> QPVNHLVKEIDMLLKEYLLSGDISEAEHCLKELEVPHFHHELVYEAIVMVLESTGESAFKMILDLLKSLWKSSTITIDQMKRGYERIYNEIPDINLDVPH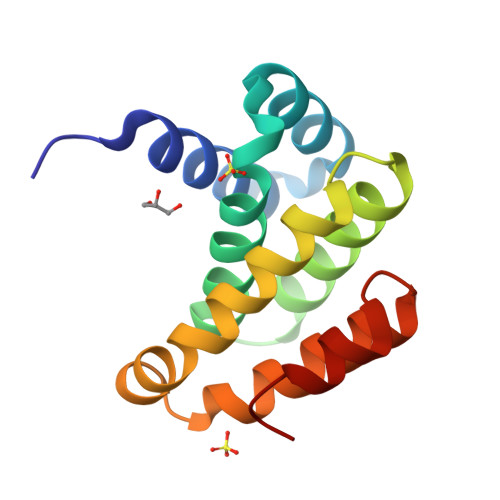SYSVLERFVEECFQAGIISKQLRDLCPSR> ASVHGTTYELLRRQGIDTVFGNPGSNELPFLKDFPEDFRYILALQEACVVGIADGYAQASRKPAFINLHSAAGTGNAMGALSNAWNSHSPLIVTAGQQTRAMIGVEALLTNVDAANLPRPLVKWSYEPASAAEVPHAMSRAIHMASMAPQGPVYLSVPYDDWDKDADPQSHHLFDRHVSSSVRLNDQDLDILVKALNSASNPAIVLGPDVDAANANADCVMLAERLKAPVWVAPSAPRCPFPTRHPCFRGLMPAGIAAISQLLEGHDVVLVIGAPVFRYHQYDPGQYLKPGTRLISVTCDPLEAARAPMGDAIVADIGAMASALANLVEESSRQLPTAAPEPAKVDQDAGRLHPETVFDTLNDMAPENAIYLNESTSTTAQMWQRLNMRNPGSYYFCAAGGLGFALPAAIGVQLAEPERQVIAVIGDGSANYSISALWTAAQYNIPTIFVIMNNGT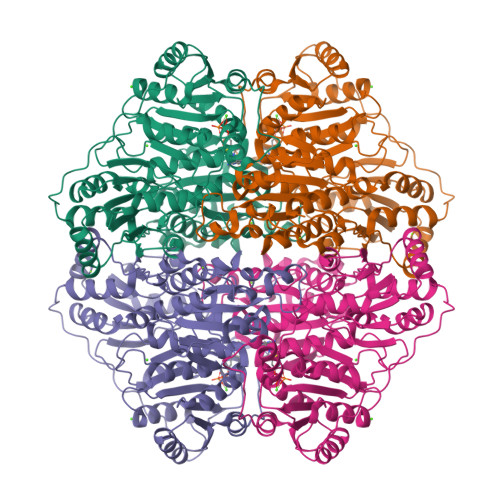YGVLRWIAGVLEAENVPGLDVPGIDFRALAKGYGVQALKADNLEQLKGSLQEALSAKGPVLIEVSTVS>MAKKIITVNVNGKAQEKAVEPRTLLIHFLREELNLTGAHIGCETSHCGACTVDIDGRSVKSCTHLAVQCDGSEVLTVEGLANKGVLHAVQEGFYKEHGL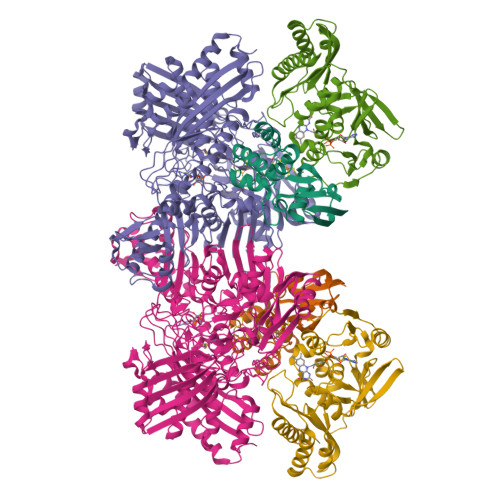QCGFCTPGMLMRAYRFLQENPNPTEAEIRMGMTGNLCRCTGYQNIVKAVQYAARKLQEPSTAAA[2x];>[2x]MNAPVQDAEARELALAGMGASRLRKEDARFIQGKGNYVDDIKMPGMLHMDIVRAPIAHGRIKKIHKDAALAMPGVHAVLTAEDLKPLKLHWMPTLAGDVAAVLADEKVHFQMQEVAIVIADDRYIAADAVEAVKVEYDELPVVIDPIDALKPDAPVLREDLAGKTSGAHGPREHHNHIFTWGAGDKAATDAVFANAPVTVSQHMYYPRVHPCPLETCGCVASFDPIKGDLTTYITSQAPHVVRTVVSMLSGIPESKVRIVSPDIGGGFGNKVGIYPGYVCAIVASIVLGRPVKWVEDRVENISTTAFARDYHMDGELAATPDGKILGLRVNVVADHGAFDACADPTKFPAGLFHICSGSYDIPRAHCSVKGVYTNKAPGGVAYRCSFRVTEAVYLIERMVDVLAQKLNMDKAEIRAKNFIRKEQFPYTTQFGFEYDSGDYHTALKKVLDAVDYPALRAEQAARRADPNSPTLMGIGLVTFTEVVGAGPSKMCDILGVGMFDSCEIRIHPTGSAIARMGTITQGQGHQTTYAQIIATELGIPSEVIQVEEGDTSTAPYGLGTYGSRSTPVAGAAIALAARKIHAKARKIAAHMLEVNENDLDWEVDRFKVKGDDSKFKTMADIAWQAYHQPPAGLEPGLEAVHYYDPPNFTYPFGIYLCVVDIDRATGETKVRRFYALDDCGTRINPMIIEGQIHGGLTEGYAVAMGQQMPFDAQGNLLGNTLMDYFLPTAVETPHWETDHTVTPSPHHPIGAKGVAESPHVGSIPTFTAAVVDAFAHVGVTHLDMPHTSYRVWKSLKEHNLAL;>MIPPRFEYHAPKSVGEAVALLGQLGSDAKLLAGGHSLLPMMKLRFAQPEHLIDINRIPELRGIREEGSTVVIGAMTVENDLISSPIVQARLPLLAEAAKLIADPQVRNRGTIGGDIAHGDPGNDHPALSIAVEAHFVLEGPNGRRTVPADGFFLGTYMTLLEENEVMVEIRVPAFAAGTGWAYEKLKRKTGDWATAGCAVVMRKSGGTVSHIRIALTNVAPTALRAEAAEAALLGKAFTKEAVQAAADAAIAICEPAEDLRGDADYKTAMAGQMVKRALNAAWARCA[2x]The covalent attachment of ubiquitin to specific protein substrates is achieved through the action of E3 ubiquitin ligases. Parkin has been proposed to function as a RBR ligase such that it encompasses both of the major classes of E3 ligase in one protein. Our structural, biochemical and cellular data indicate that Parkin functions as a RING/HECT hybrid. Parkin likely binds E2 through a conserved structural motif on a canonical RING domain, and also functions through a HECT-like active site cysteine whose activity can be regulated through interaction between the R0 and R2 domains.

To gain insight into the RBR class of E3 ligase, we grew crystals of Parkin-R0RBR (residues 141–465) that includes RING 0 (R0) and the RBR domains. The structure was determined by analysis of multiwavelength anomalous diffraction data using the signal from Zn ions bound by the individual RING domains and was refined against high resolution data to 1.58 Å. Our 1.58 Å structure reveals that Parkin forms a relatively compact overall structure with multiple unpredicted domain interfaces. We solved two structures of Parkin to determine if there were any notable structural differences between the sequence of Parkin originally reported (containing P223) and the updated sequence (S223). Overall the two structures were extremely similar; however, the loop containing S223 was visible in Parkin-R0RBR but not in the P223 structure. Aspects discussed in this paper were indistinguishable for Parkin with S or P at position 223; The structure discussion focuses on the S223 protein. Each RING domain binds two Zn ions and resolves discrepancies in the literature regarding Zn coordination. The R0RBR structure reveals that the molecule is folded in half with the N- and C-termini forming an extensive interface that comprise two compact domain groups separated by two linkers. One domain group is comprised of an association between R1 and IBR, the other domain group is formed by a close association of R0 and R2. In our structure, H433 is involved in water-mediated hydrogen bonding with W462 and is not available to deprotonate C431, representing an inactive state of the enzyme through misalignment of the catalytic residues.

> SIYNSFYVYCKGPCQRVQPGKLRVQCSTCRQATLTLTQGPSCWDDVLIPNRMSGECQSPHCPGTSAEFFFKCGAHPTSDKETPVALHLIATNSRNITCITCTDVRSPVLVFQCNSRHVICLDCFHLYCVTRLNDRQFVHDPQLGYSLPCVAGCPNSLIKELHHFRILGEEQYNRYQQYGAEECVLQMGGVLCPRPGCGAGLLPEPDQRKVTCEGGNGLGCGFAFCRECKEAYHEGECSAVFEASGTTTQAYRVDERAAEQARWEAASKETIKKTTKPCPRCHVPVEKNGGCMHMKCPQPQCRLEWCWNCGCEWNRVCMGDHWFDV N-acetyl-L-leucyl-N-[(4S,5S,7R)-8-(butylamino)-5-hydroxy-2,7-dimethyl-8-oxooctan-4-yl]-L-methioninamide | C27 H52 N4 O5 S | 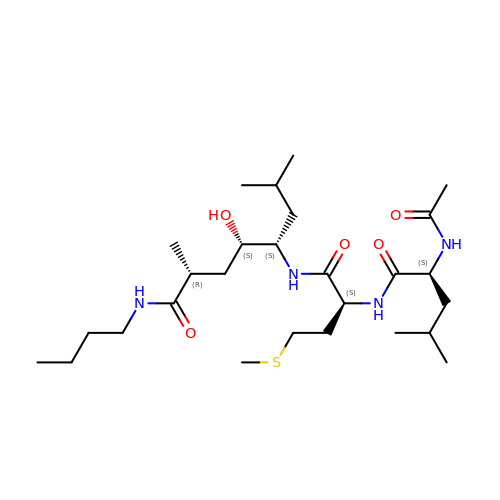PEWRQHFGBBTOMS-FFYZIMEISA-N> AVGIFVIIFGIALFFLAMKVSGLVGTNLSDGYTMKAQFDNVNGLKPRAKVTMSGVTIGRVDSITLDPVTRLATVTFDLDGKLTSFNAEQLKEVQKNA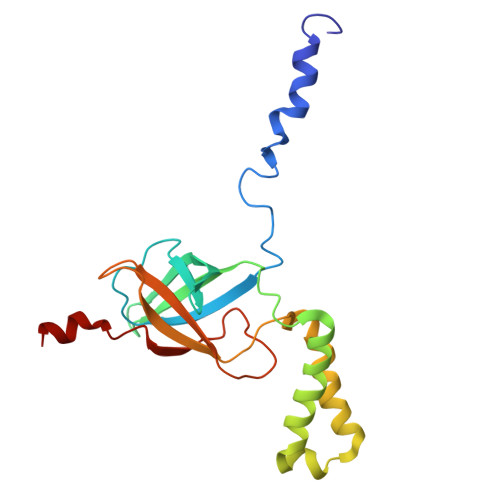LDELRYSSDYTQATPAQQKTMEQQLISNMNSITSIDEDAYIMVATNGLLGEKYLKIVPGGGLNYLKRGDTISNTQGTMDLEDLISK>[4x]MNAKEIVVHALR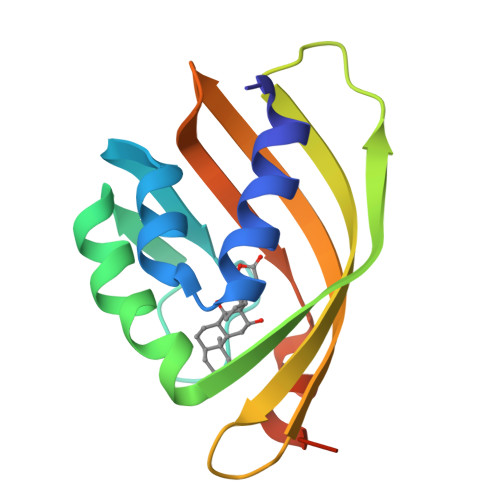LLENGDARGWCDLFHPEGVLEYPYPPPGYKTRFEGRETIWAHMRLFPEYMTIRFTDVQFYETADPDLAIGEFHGDGVHTVSGGKLAADYISVLRTRDGQILLYRLFFNPLRVLEPLGLEHHHHHH>GQDMVSPPPPIADEPLTVNTGIYLIECYSLDDKAETFKVNAFLSLSWKDRRLAFDPVRSGVRVKTYEPEAIWIPEIRFVNVENARDADVVNISVSPDGTVQYLERFSARVLSPLDFRRYPFDSQTLHIYLIVRSVDTRNIVLAVDLEKVGKNDDVFLTGWDIESFTAVVKPANFALQNRLESKLDYQLRISRQYFSYIPNIILPMLFILFISWTAFWSTSYEANVTLVVSTLIAHIAFNILVETNLPKTPYMTYTGAIIFMIYLFYFVAVIEVTVQHYLKVESQPARAASITRASRI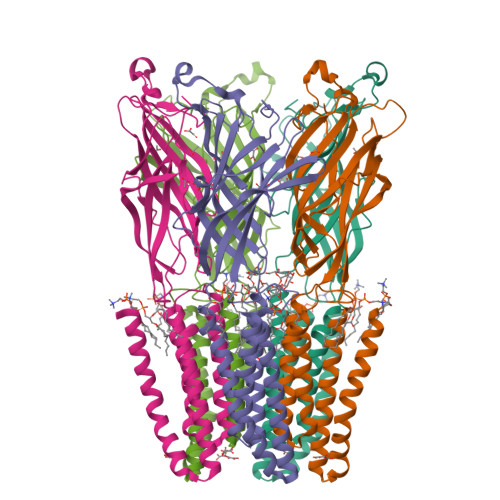AFPVVFLLANIILAFLFFGF[5x]>[2x]HHHHHHAGAEGALIRFYVEIEELIYIDVFTTRPDTVFGATFVVLAPEHPLVPVLACIGERLGNACYSDVENFVEKMKKMSTRERTMEEDKEGVFLGVYATNPANGEK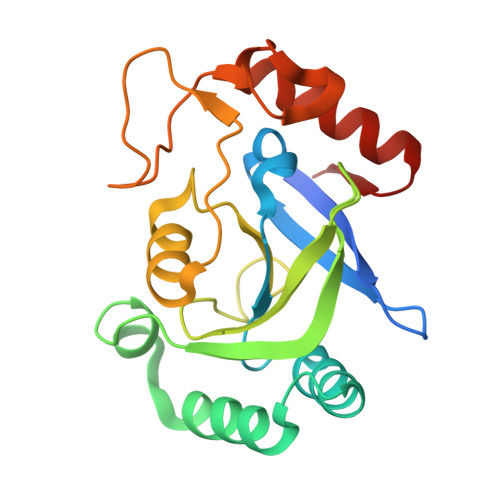IPVWSANYVLYEYGTGAIMCVPAHDQRDWEFAKKYDLPIKVVVKPEGAWDFEKGAYEGKGTLVNSDGFDGLDSETAKRKITEWLQDRGLGEKKV>[2x]MSYYHHHHHHDYKDDDDKLEVLFQGPEFMPAPRAREQPRVPGERQPLLPRGARGPRRWRRAAGAAVLLVEMLERAAFFGVTANLVLYLNSTNFNWTGEQATRAALVFLGASYLLAPVGGWLADVYLGRYRAVALSLLLYLAASGLLPATAFPDGRSSFCGEMPASPLGPACPSAGCPRSSPSPYCAPVLYAGLLLLGLAASSVRSNLTSFGADQVMDLGRDATRRFFNWFYWSINLGAVLSLLVVAFIQQNISFLLGYSIPVGCVGLAFFIFLFATPVFITKPPMGSQVSSMLKLALQNCCPQLWQRHSARDRQCARVLADERSPQPGASPQEDIANFQVLVKILPVMVTLVPYWMVYFQMQSTYVLQGLHLHIPNIFPANPANISVALRAQGSSYTIPEAWLLLANVVVVLILVPLKDRLIDPLLLRCKLL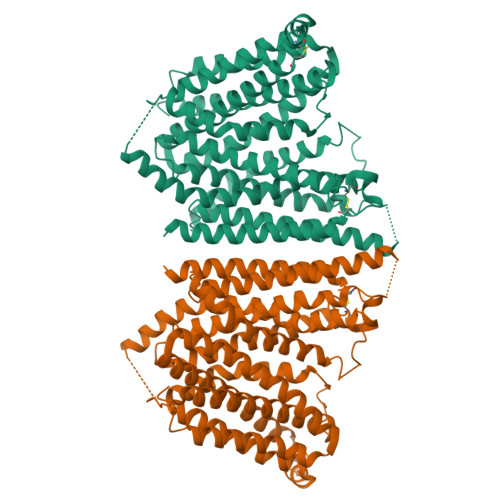PSALQKMALGMFFGFTSVIVAGVLEMERLHYIHHNETVSQQIGEVLYNAAPLSIWWQIPQYLLIGISEIFASIPGLEFAYSEAPRSMQGAIMGIFFCLSGVGSLLGSSLVALLSLPGGWLHCPKDFGNINNCRMDLYFFLLAGIQAVTALLFVWIAGRYERASQGPASHSRFSRDRG2,2-dimethylpropanoyloxymethyl (2R)-5-(aminocarbonyloxymethyl)-2-[(1R)-1-[[(Z)-2-(2-azanyl-1,3-thiazol-4-yl)pent-2-enoyl]amino]-2-oxidanylidene-ethyl]-3,6-dihydro-2H-1,3-thiazine-4-carboxylate 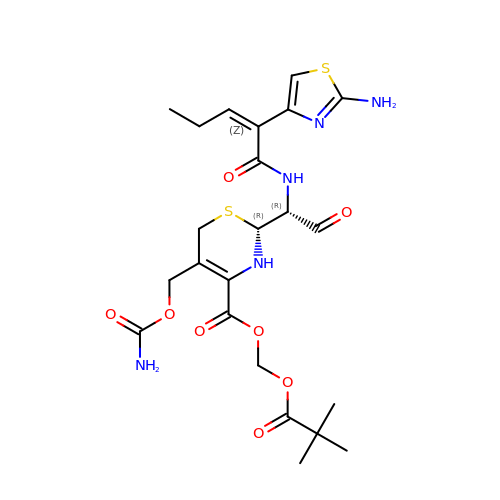| C23 H31 N5 O8 S2 | CXZSGDIZUNIAQH-FJWVKOTRSA-N> HHHHHHHHGSSTSNIEGRSRVTRDCVQRCIVEEDLFLDEFGIQCEKADNGEKCYKTRCTKGCAQWYRALKELESCQEACLSLQFYPYDMPCIGACEMAQRDYWHLQRLAISHLVERTQPQLERAPRADGQSTPLTIRWAMHFPEHYLASRPFNIQYQFVDHHGEELDLEQEDQDASGETGSSAWFNLADYDCDEYYVCEILEALIPYTQYRFRFELPFGENRDEVLYSPATPAYQTPPEGAPISAPVIEHLMGLDDSHLAVHWHPGRFTNGPIEGYRLRLSSSEGNATSEQLVPAGRGSYIFSQLQAGTNYTLALSMINKQGEGPVAKGFVQTHSARNEKPAKDLTESVLLVGRRAVMWQSLEPAGENSMIYQSQEELADIAWSKREQQLWLLNVHGELRSLKFESGQMVSPAQQLKLDLGNISSGRWVPRRLSFDWLHHRLYFAMESPERNQSSFQIIS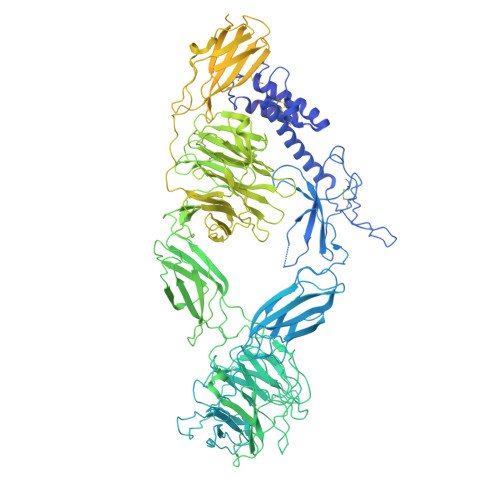TDLLGESAQKVGESFDLPVEQLEVDALNGWIFWRNEESLWRQDLHGRMIHRLLRIRQPGWFLVQPQHFIIHLMLPQEGKFLEISYDGGFKHPLPLPPPSNGAGNGPASSHWQSFALLGRSLLLPDSGQLILVEQQGQAASPSASWPLKNLPDCWAVILLVPESQPLTSAGGKPHSLKALLGAQAAKISWKEPERNPYQSADAARSWSYELEVLDVASQSAFSIRNIRGPIFGLQRLQPDNLYQLRVRAINVDGEPGEWTEPLAARTWPLGPHRLRWASRQGSVIHTNELGEGLEVQQEQLERLPGPMTMVNESVGYYVTGDGLLHCINLVHSQWGCPISEPLQHVGSVTYDWRGGRVYWTDLARNCVVRMDPWSGSRELLPVFEANFLALDPRQGHLYYATSSQLSRHGSTPDEAVTYYRVNGLEGSIASFVLDTQQDQLFWLVKGSGALRLYRAPLTAGGDSLQMIQQIKGVFQAVPDSLQLLRPLGALLWLERSGRRARLVRLAAPLDVMELPTPDQASPASALQLLDPQPLPPRDEGVIPMTVLPDSVRLDDGHWDDFHVRWQPSTSGGNHSVSYRLLLEFGQRLQTLDLSTPFARLTQLPQAQLQLKISITPRTAWRSGDTTRVQLTTPPVAPSQPRRLRVFVERLATALQEANVSAVLRWDAPEQGQEAPMQALEYHISCWVGSELHEELRLNQSALEARVEHLQPDQTYHFQVEARVAATGAAAGAASHALHVAPEVQAVPRVLYANAEFIGELDLDTRNRRRLVHTASPVEHLVGIEGEQRLLWVNEHVELLTHVPGSAPAKLARMRAEVLALAVDWIQRIVYWAELDATAPQAAIIYRLDLCNFEGKILQGERVWSTPRGRLLKDLVALPQAQSLIWLEYEQGSPRNGSLRGRNLTDGSELEWATVQPLIRLHAGSLEPGSETLNLVDNQGKLCVYDVARQLCTASALRAQLNLLGEDSIAGQLAQDSGYLYAVKNWSIRAYGRRRQQLEYTVELEPEEVRLLQAHNYQAYPPKNCLLLPSSGGSLLKATDCEEQRCLLNLPMITASEDCPLPIPGVRYQLNLTLARGPGSEEHDHGVEPLGQWLLGAGESLNLTDLLPFTRYRVSGILSSFYQKKLALPTLVLAPLELLTASATDYKDDDDK> AFDGTWKVDRNENYEKFMEKMGINVVKRKLGAHDNLKLTITQEGNKFTVKESSNFRNIDNVFELGVDFAYSLADGTELTGTWTMEGNKLVGKFKRVDNGKELIAVREISGNELIQTYTYEG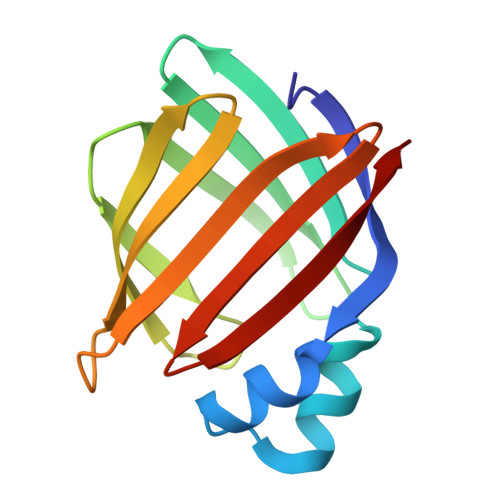VEAKRIFKKE> MGAAAKLAFAVFLISCSSGAILGRSETQECLFFNANWEKDRTNQTGVEPCYGDKDKRRHCFATWKNISGSIE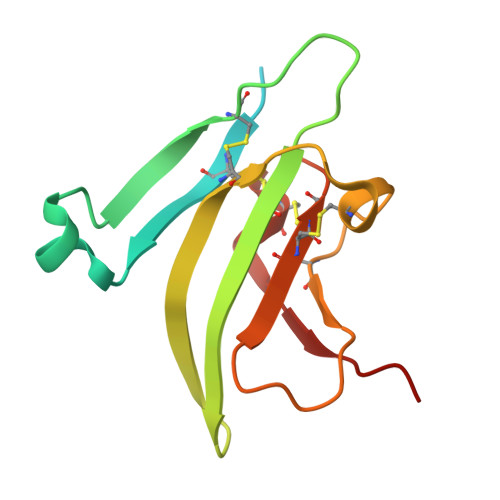IVKQGCWLDDINCYDRTDCVEKKDSPEVYFCCCEGNMCNEKFSYFPEME Alkaline phosphatases (EC 3.1.3.1) hereafter referred to as APs, are widely distributed enzymes that hydrolyze the phosphate monoesters under alkaline pH conditions. Recently we reported extraction of an AP, termed SPAP, from the bacterium Sphingomonas sp. strain BSAR-1, exhibiting several unique features, such as constitutive expression, thermo-lability, extracellular release and high specific activity. SPAP requires Ca2+ and Zn2+ for activity, while magnesium has no effect. In conclusion, three dimensional structure of a substrate-bound alkaline phosphatase (SPAP) from the Sphingomonas sp. strain BSAR -1 bacterium has been determined to a resolution of 1.95 Å.

The final contents of the asymmetric unit are: 526 protein residues (31–556), two zinc ions of partial occupancy (0.75), 278 water molecules, 5 glycerol molecules, 1 Ca2+ ion and one organic phosphate in the active site. The overall shape of the protein can be described as that of a shallow cup with a thick base. The two active-site metal ions (M1 and M2), which were identified as Zn2+ through X-ray fluorescence measurements, are 4.1 Å apart. Zn2+ ion at M1 site is in coordination to polar atoms from His 491, His 304 and Asp 300, while Zn2+ at M2 site is coordinated by His346, Thr89, Asp345 and Asp49. Structural superposition confirmed the catalytic residue in SPAP as Thr89, which was also suggested by sequence alignment. Unaccounted electron density was observed in the active site region, and the volume of this density is larger than that for an inorganic phosphate, and therefore, we have interpreted this density to represent a phosphomonoester, ROPO3, substrate. One of the nonbridging phosphate oxygens, O3, is sequestered between the two zinc ions, while the remaining two, O1 and O2, interact with residues Thr89, Arg173, Asn110 and Lys171 in the active site. In SPAP, the corresponding torsion angle is −60°, and the hydroxyl of Thr89 is pointing toward the phosphate, thus confirming that the present structure is not a product complex, but is a Michaelis complex relevant to the first stage in which the phosphoenzyme is formed. The residues Thr155 and Glu322 in ECAP are replaced by Ala174 and Gly295 respectively in SPAP. These changes abolished the third metal coordination site, and therefore there is no third metal bound to SPAP inthe active site. Interestingly, a lysine residue is recruited into the active site of SPAP, and the position of this residue is such that the positively charged NZ atom almost overlaps the water molecule coordinating the Mg2+ ion in the ECAP structure.

> MLKHVAAALLLATAMPVVAQSPAPAAAPAPAARSIAATPPKLIVAISVDQFSADLFSEYRQYYTGGLKRLTSEGAVFPRGYQSHAATETCPGHSTILTGSRPSRTGIIANNWFDLDAKREDKNLYCAEDESQPGSSSDKYEASPLHLKVPTLGGRMKAANPATRVVSVAGKDRAAIMMGGATADQVWWLGGPQGYVSYKGVAPTPLVTQVNQAFAQRLAQPNPGFELPAQCVSKDFPVQAGNRTVGTGRFARDAGDYKGFRISPEQDAMTLAFAAAAIENMQLGKQAQTDIISIGLSATDYVGHTFGTEGTESCIQVDRLDTELGAFFDKLDKDGIDYVVVLTADHGGHDLPERHRMNAMPMEQRVDMALTPKALNATIAEKAGLPGKKVIWSDGPSGDIYYDKGLTAAQRARVETEALKYLRAHPQVQTVFTKAEIAATPSPSGPPESWSLIQEARASFYPSRSGDLLLLLKPRVMSIPEQAVMGSVATHGSPWDTDRRVPILFWRKGMQHFEQPLGVETVDILPSLAALIKLPVPKDQIDGRCLDLVAGKDDSCAGQHHHHHH(1S)-2-{[(2-AMINOETHOXY)(HYDROXY)PHOSPHORYL]OXY}-1-[(PALMITOYLOXY)METHYL]ETHYL 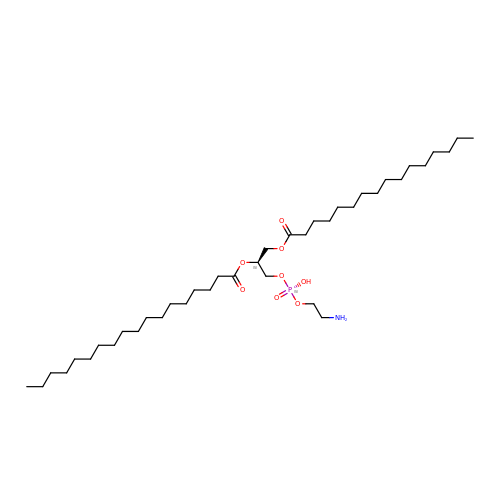STEARATE | C39 H78 N O8 P | RPJZYOHZALDGKI-QNGWXLTQSA-N> GAGRHPPVVLVPGDLGNQLEAKLDKPTVVHYLCSKKTESYFTIWLNLELLLPVIIDCWIDNIRLVYNKTSRATQFPDGVDVRVPGFGKTFSLEFLDPSKSSVGSYFHTMVESLVGWGYTRGEDVRGAPYDWRRAPNENGPYFLALREMIEEMYQLYGGPVVLVAHAMGNMYTLYFLQRQPQAWKDKYIRAFVSLGAPWGGVAKTLRVLASGDNNRIPVIGPLKIREQQRSAVSTSWLLPYNYTWSPEKVFVQTPTINYTLRDYRKFFQDIGFEDGWLMRQDTEGLVEATMPPGVQLHCLYGTGVPTPDSFYYESFPDRDPKICFGDGDGTVNLKSALQCQAWQSRQEHQVLLQELPGSEHIE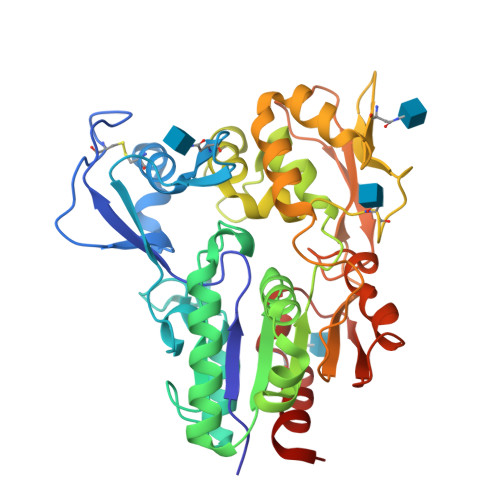MLANATTLAYLKRVLLGP> CCAACGTT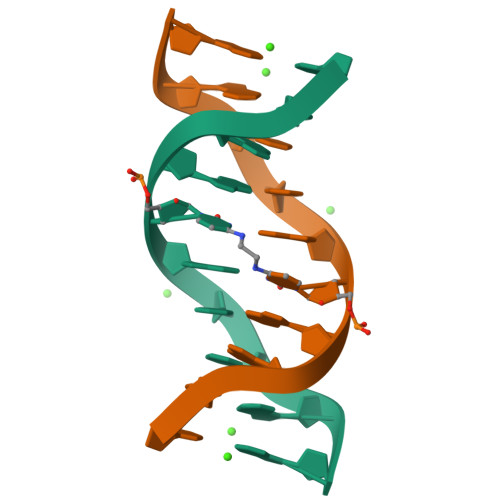GG>[4x]MTSASNPPAFRLETSDGDEEGSAEVNKGKNEPPPMESPFQGEDRNFSPQIKVNLNYRKGLGPSQQDPNRFDRDRLFSVVSRGVPEELTGLLEYLRRTSKYLTDSAYTEGSTGKTCLMKAVLNLQDGVNACILPLLQIDRDSGNPQPLVNAQCTDEFYRGHSALHIAIEKRSLWCVKLLVENGANVHIRACGRFFQKHQGTCFYFGELPLSLAACTKQWDVVTYLLENPHQPASLEATDSLGNTVLHALVMIADNSPENSALVIHMYDSLLQMGARLCPTVQLEDICNHQGLTPLKLAAKEGKIEIFRHILQREFSGLYQPLSRKFTEWCYGPVRVSLYDLS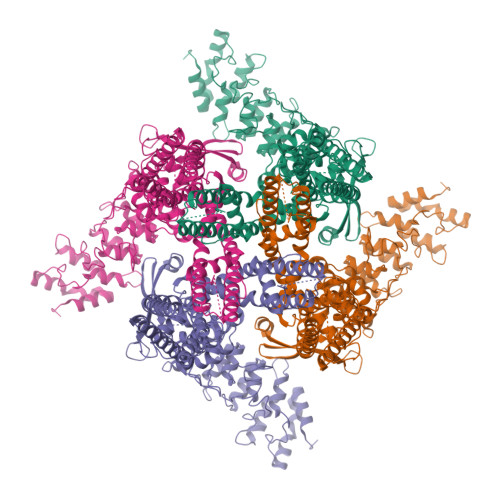SVDSWEKNSVLEIIAFHCKSPHRHRMVVLEPLNKLLQEKWDRLIPRFFFNFACYLVYMIIFTIVAYHQPSLEQPAIPSSKATFGDSMLLLGHILILLGGIYLLLGQLWYFWRRRLFIWISFMDSYFEILFLVQALLTVLSQVLRFVETEWYLPLLVSSLVLGWLNLLYYTRGFQHTGIYSVMIFKVILRDLLRFLLVYLVFLFGFAVALVSLSREARSPKAPEDSNTTVTEKPTLGQEEEPVPYGGILDASLELFKFTIGMGELAFQEQLRFRGVVLLLLLAYVLLTYVLLLNMLIALMSETVNSVATDSWSIWKLQKAISVLEMENGYWWCRRKRHRAGRLLKVGTKGDGIPDERWCFRVEEVNWAAWEKTLPTLSEDPSGAGITGYKKNPTSKPGKNSASEEDHLPLQVLQSH>MSESPLRLDRLRDFVSALGELLDRHPDEESVL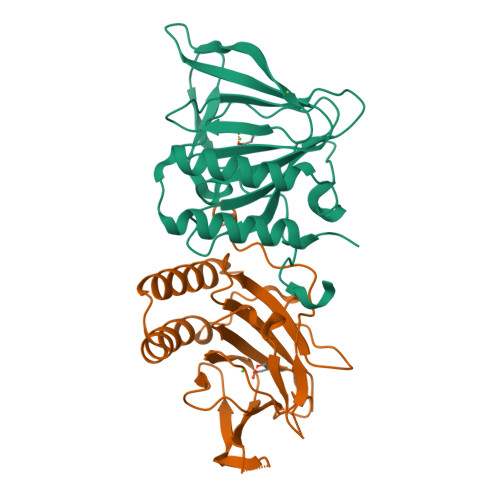REGRSLLGELVRHDDWLPEEFAQPDPERYQQYLLHADSRQRFSVVSFVWGPGQTTPVHDHRVWGLIGMLRGAEDAQSFELGAEGLRPIGDPVRLSPGQVEAVSPRIGDIHRVFNASPDQPSISIHVYGANIGAVRRAVYLPDGSEKPFISGYSNQFLPNIWDQSKESARPVDLVPR[12x]>MKVLVTGFEPFGGEKINPTERIAKDLDGIKIGDAQVFGRVLPVVFGKAKEVLEKTLEEIKPDIAIHVGLAPGRSAISIERIAVNAIDARIPDNEGKKIEDEPIVPGAPTAYFSTLPIKKIMKKLHERGIPAYISNSAGLYLCNYVMYLSLHHSATKGYPKMSGFIHVPYIPEQIIDKIGKGQVPPSM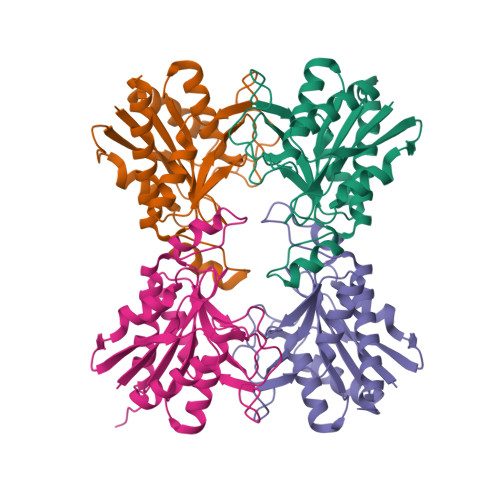CYEMELEAVKVAIEVALTQDMINKST[4x]>[2x]MTTATAGLAVELKQSTAQAHEKAEHSTFMSDLLKGRLGVAEFTRLQEQAWLFYTALEQAVDAVRASGFAESLLDPALNRAEVLARDLDKLNGSS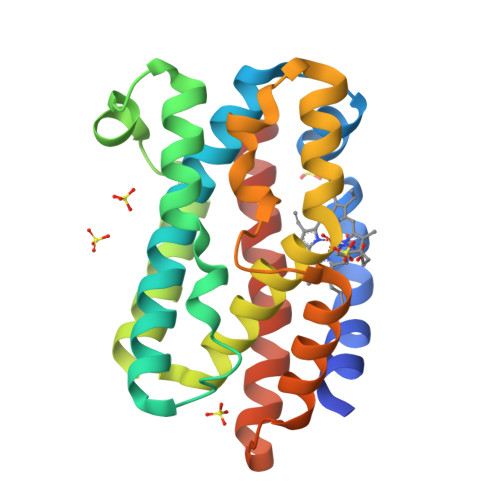EWRSRITASPAVIDYVNRLEEIRDNVDGPALVAHHYVRYLGELSGGQVIARMMQRHYGVDPEALGFYHFEGIAKLKVYKDEYREKLNNLELSDEQREHLLKEATDAFVFNHQVFADLGKGL>APQDPRNLPIRQQMEALIRRKQAEITQGLESIDTVKFHADTWTRGNDGGGGTSMVIQDGTTFEKGGVNVSVVYGQLSPAAVSAMKADHKNLRLPEDPKTGLPVTDGVKFFACGLSMVIHPVNPHAPTTHLNYRYFETWNQDGTPQTWWFGGGADLTPSYLYEEDGQLFHQLHKDALDKHDTALYPRFKKWCDEYFYITHRKETRGIGGIFFDDYDERDPQEILKMVEDCFDAFLPSYLTIVKRRKDMPYTKEEQQWQAIRRGRYVEFNLIYDRGTQFGL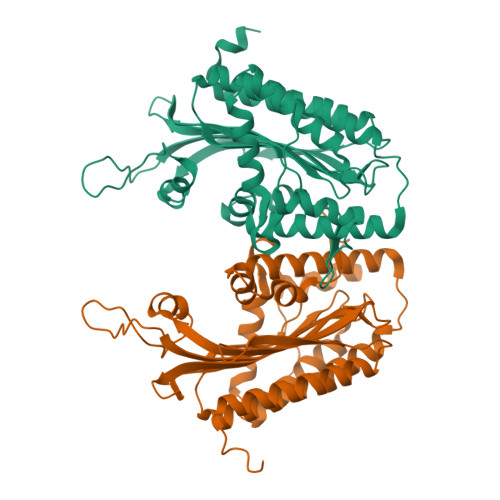RTPGSRVESILMSLPEHASWLYNHHPAPGSREAKLLEVTTKPREWVK[2x]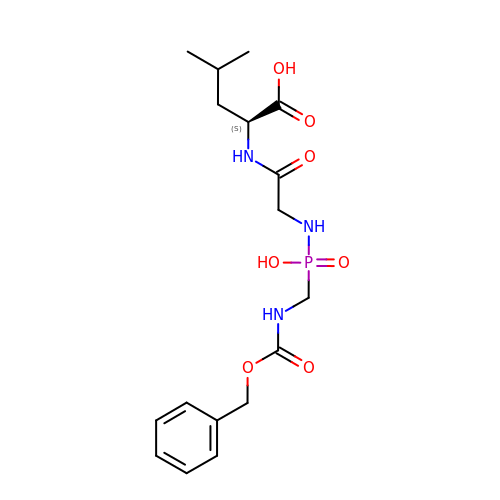(2~{S})-4-methyl-2-[2-[[oxidanyl(phenylmethoxycarbonylaminomethyl)phosphoryl]amino]ethanoylamino]pentanoic acid | C17 H26 N3 O7 P | MOYNPRDFZGMZHZ-AWEZNQCLSA-N>MNKQEVILKVQECAAWWILERQSKLTKLMSETMSINPFMTPFIFDYHSLNDFDELVEAIIAKHLMTGHDTGFGKLIDEKILPRVFGAYKLDKSYRAANEPFIHPCFDEIDHVIQRDDGRIELLSLKAGKWTIQLTMAVQLNKAFHEIINNYPGVADNIVVGVFYGNSHGLTDKYRILRGINTGANHNVIDIRDKVHVYAGKEFWSWLNNGEAETQHWVLEGIERAVKEADIKEKNKDLIEKFKEHVAKKYNEQVLNADGTAQWHKLLEMINE[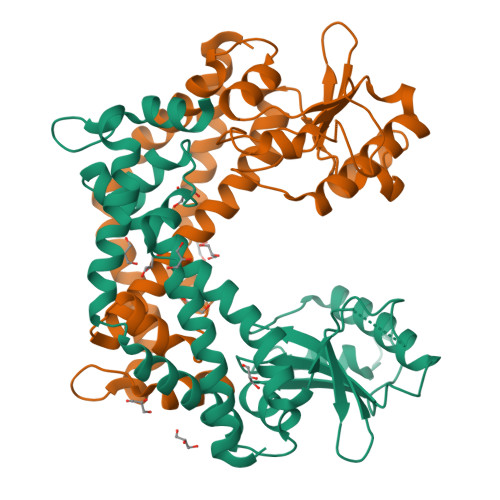2x]> MIYLRKANERGHANHGWLDSWHTFSFANYYDPNFMGFSALRVINDDVIEAGQGFGTHPHKDMEILTYVLEGTVEHQDSMGNKEQVPAGEFQIMSAGTGIRHSEYNPSST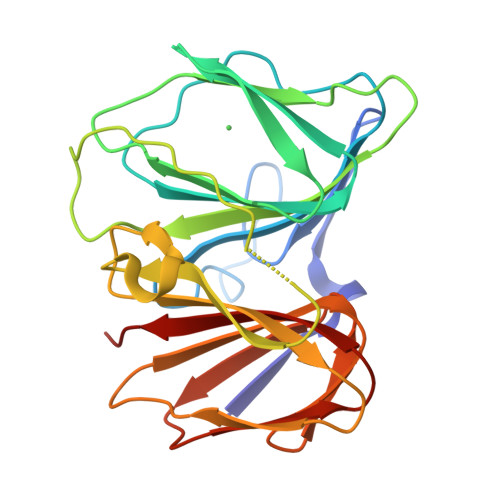ERLHLYQIWIMPEENGITPRYEQRRFDAVQGKQLVLSPDARDGSLKVHQDMELYRWALLKDEQSVHQIAAERRVWIQVVKGNVTINGVKASTSDGLAIWDEQAISIHADSDSEVLLFDLPPV>AMAELKEFLNKPAATSDVPPAPAGFDFDAAKKLVDVRCNKCHTLDSVADLFRTKYKKTGQVNLIVKRMQ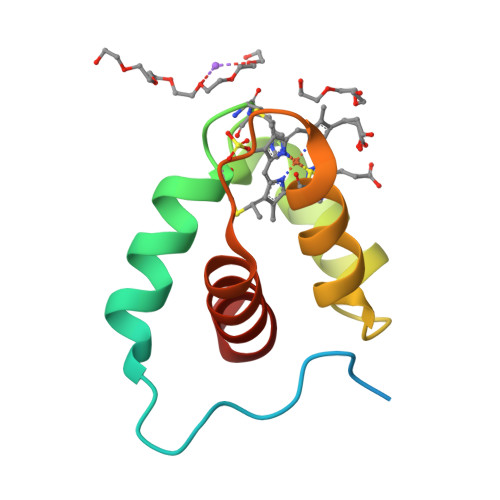GFPGSGISDDDAKTIGIWLHEKF[2x]> MAQIDFRKKINWHRRYRSPQGVKTEHEILRIFESDRGRIINSPAIRRLQQKTQVFPLERNAAVRTRLTHSMEVQQVGRYIAKEILSRLKELKLLEAYGLDELTGPFESIVEMSCLMHDIGNPPFGHFGEAAINDWFRQRLHPEDAESQPLTDDRCSVAALRLRDGEEPLNELRRKIRQDLCHFEGNAQGIRLVHTLMRMNLTWAQVGGILKYTRPAWWRGETPETHHYLMKKPGYYLSEEAYIARLRKELNLALYSRFPLTWIMEAADDISYCVADLEDAVEKRIFTVEQLYHHLHEAWGQHEKGSLFSLVVENAWEKSRSNSLSRSTEDQFFMYLRVNTLNKLVPYAAQRFIDNLPAIFAGTFNHALLEDASECSDLLKLYKNVAVKHVFSHPDVERLELQGYRVISGLLEIYRPLLSLSLSDFTELVEKERVKRFPIESRLFHKLSTRHRLAYVEAVSKLPSDSPEFPLWEYYYRCRLLQDYISGMTDLYAWDEYR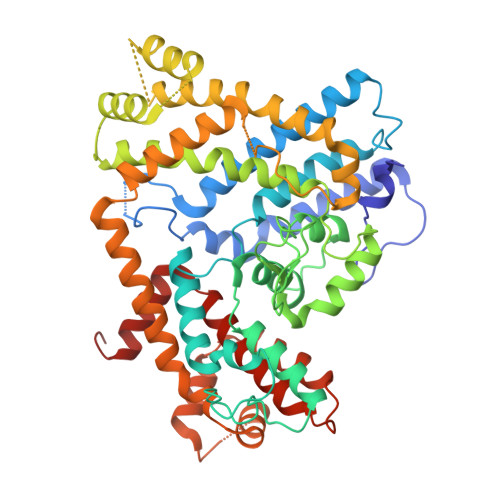RLMAVEQ>[2x]TCRYLLVRSLQTFSQ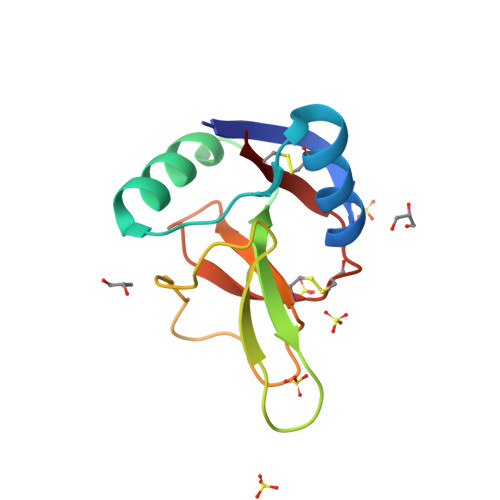AWFTCRRCYRGNLVSIHNFNINYRIQCSVSALNQGQVWIGGRITGSGRCRRFQWVDGSRWNFAYWAAHQPWSRGGHCVALCTRGGYWRRAHCLRRLPFICSY> MARQNLKSTDRAVQQMLDKAKREGIQTVWDRYEAMKPQCGFGETGLCCRHCLQGPCRINPFGDEPKVGICGATAEVIVARGLDRSIAAGAAGASGHAKHLAHTLKKAVQGKAASYMIKDRTKLHSIAKRLGIPTEGQKDEDIALEVAKAALADFHEKDTPVLWVTTVLPPSRVKVLSAHGLIPAGIDHEIAEIMHRTSMGCDADAQNLLLGGLRCSLADLAGCYMGTDLADILFGTPAPVVTESNLGVLKADAVNVAVHGHNPVLSDIIV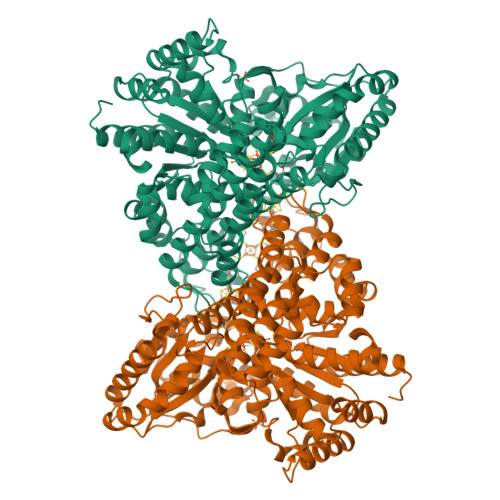SVSKEMENEARAAGATGINVVGICCTGNEVLMRHGIPACTHSVSQEMAMITGALDAMILDYQCIQPSVATIAECTGTTVITTMEMSKITGATHVNFAEEAAVENAKQILRLAIDTFKRRKGKPVEIPNIKTKVVAGFSTEAIINALSKLNANDPLKPLIDNVVNGNIRGVCLFAGCNNVKVPQDQNFTTIARKLLKQNVLVVATGCGAGALMRHGFMDPANVDELCGDGLKAVLTAIGEANGLGGPLPPVLHMGSCVDNSRAVALVAALANRLGVDLDRLPVVASAAEAMHEKAVAIGTWAVTIGLPTHIGVLPPITGSLPVTQILTSSVKDITGGYFIVELDPETAADKLLAAINERRAGLGLPW>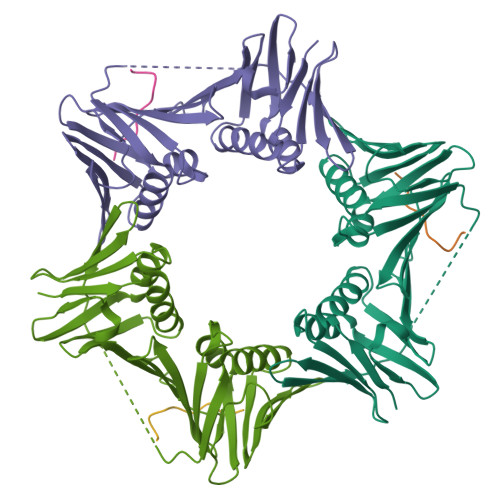 MRGSHHHHHHGSMPFEIVFEGAKEFAQLIETASRLIDEAAFKVTEEGISMRAMDPSRVVLIDLNLPASIFSKYEVDGEETIGVNMDHLKKVLKRGKAKETLILRKGEENFLEISLQGTATRTFKLPLIDVEEIEVDLPELPFTAKVVILGDVIKEAVKDASLVSDSMKFIAKENEFTMRAEGETQEVEVKLTLEDEGLLDIEVQEETKSAYGISYLSDMVKGLGKADEVTIKFGNEMPMQMEYYIRDEGRLIFLLAPRVEE;> KKRVISLEEFFS> MSGPERITLAMTGASGAQYGLRLLDCLVQEEREVHFLISKAA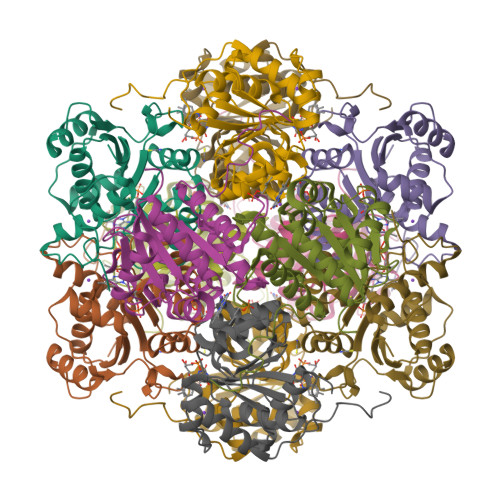QLVMATQTDVALPAKPQAMQAFLTEYCGAAAGQIRVFGQNDWMAPPASGSSAPNAMVICPCSTGTLSAVATGACNNLIERAADVALKERRPLVLVPREAPFSSIHLENMLKLSNLGAVILPAAPGFYHQPQSVEDLVDFVVARILNTLGIPQDMLPRWGEQHLVSDE> MWYKYFSKQSWNLRVWRKANLKYNQDDFGMTQPKYIARFGDFRFRLVRTEGALRGCMFFVGFGCFSIINYLYGRYGYIINESSQKRAAQDLLDNDMAADKILFKNRVGA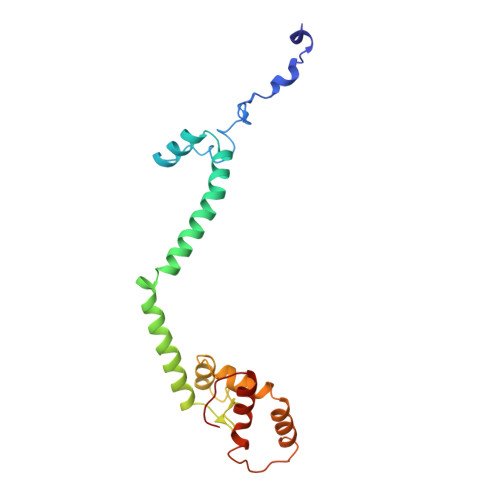PTRPLRSLDDMMAFLSGSATYDQLADYASYNHAMDVNQDQQAGLDSWMSEKDKNMVKYYQRSLGKKVEGI> GPLGSMAGMVDFQDEEQVKSFLENMEVECNYHCYHEKDPDGCYRLVDYLEGIRKNFDEAAKVLKFNCEENQHSDSCYKLGAYYVTGKGGLTQDLKAAARCFLMACEKPGKKSIAACHNVGLLAHDGQVNEDGQPDLGKARDYYTRACDGGYTSSCFNLSAMFLQGAPGFPKDMDLACKYS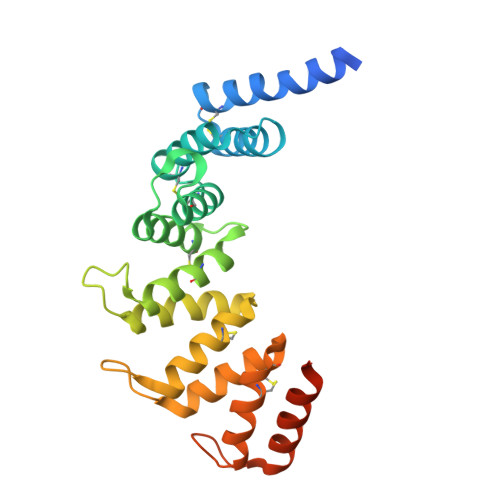MKACDLGHIWACANASRMYKLGDGVDKDEAKAEVLKNRAQQLHKEQQKGVQPLTFG>MHHHHHHELYLDTSDVVAVKALSRIFPLAGVTTNPSIIAAGKKPLDVVLPQLHEAMGGQGRLFAQVMATTAEGMVNDALKLRSIIADIVVKVPVTAEGLAAIKMLKAEGIPTLGTAVYGAAQGLLSALAGAEYVAPFVNRIDAQGGSGIQTVTDLHQLLKMHAPQAKVLAA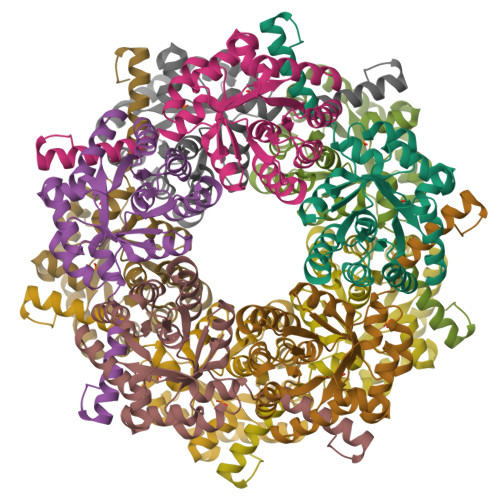SFKTPRQALDCLLAGCESITLPLDVAQQMISYPAVDAAVAKFEQDWQGAFGRTSI[10x]> AYNP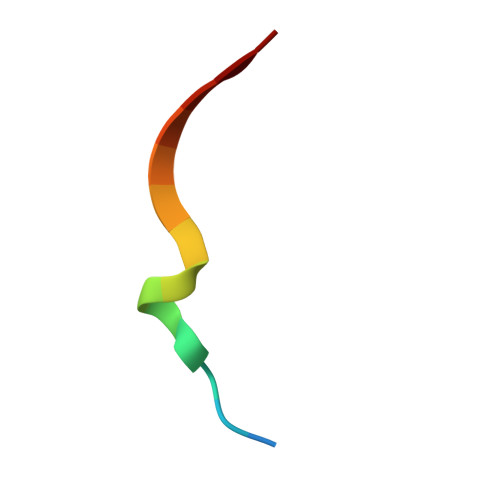YPEDYGDIEIG> MNPIHDRTSDYHKYLKVKQGDSDLFKLTVSDKRYIWYNPDPKERDSYECGEIVSETSDSFTFKTVDGQDRQVKKDDANQRNPIKFDGVEDMSELSYLNEPAVFHNLRVRYNQDLIYTYSGLFLVAVNPFKRIPIYTQEMVDIFKGRRRNEVAPHIFAISDVAYRSMLDDRQNQSLLITGESGAGKTENTKKVIQYLASVAGRNQANGSGVLEQQILQANPILEAFGNAKTTRNNNSSRFGKFIEIQFNSAGFISGASIQSYLLEKSRVVFQSETERNYHIFYQLLAGATAEEKKALHLAGPESFNYLNQSGCVDIKGVSDSEEFKITRQAMDIVGFSQEEQMSIFKIIAGILHLGNIKFEKGAGEGAVLKDKTALNAASTVFGVNPSVLEKALMEPRILAGRDLVAQHLNVEKSSSSRDALVKALYGRLFLWLVKKINNV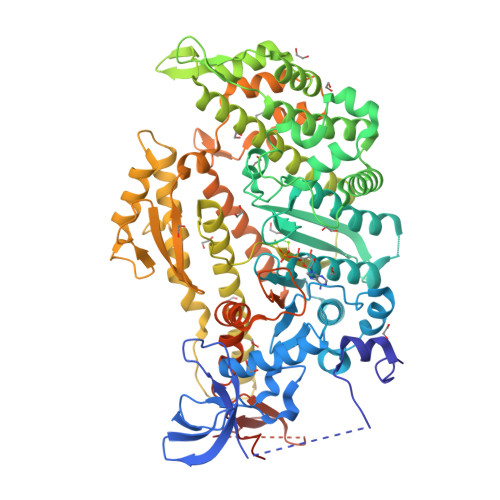LCQERKAYFIGVLDIYGFEIFKVNSFEQLCINYTNEKLQQFFNHHMFKLEQEEYLKEKINWTFIDFGLDSQATIDLIDGRQPPGILALLDEQSVFPNATDNTLITKLHSHFSKKNAKYEEPRFSKTEFGVTHYAGQVMYEIQDWLEKNKDPLQQDLELCFKDSSDNVVTKLFNDPNIASRAKKGANFITVAAQYKEQLASLMATLETTNPHFVRCIIPNNKQLPAKLEDKVVLDQLRCNGVLEGIRITRKGFPNRIIYADFVKRYYLLAPNVPRDAEDSQKATDAVLKHLNIDPEQFRFGITKIFFRAGQLARIEEARELRGDYKDDDDK>[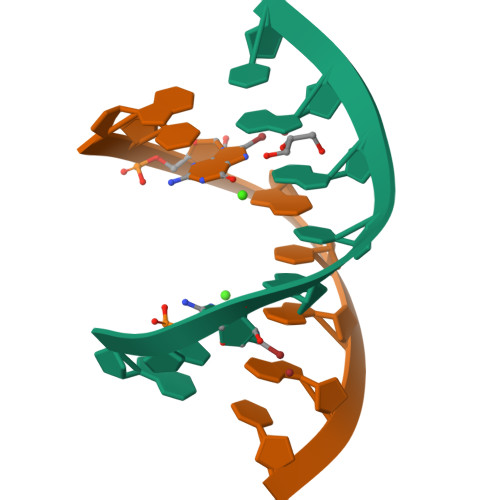2x]GCXGCGGC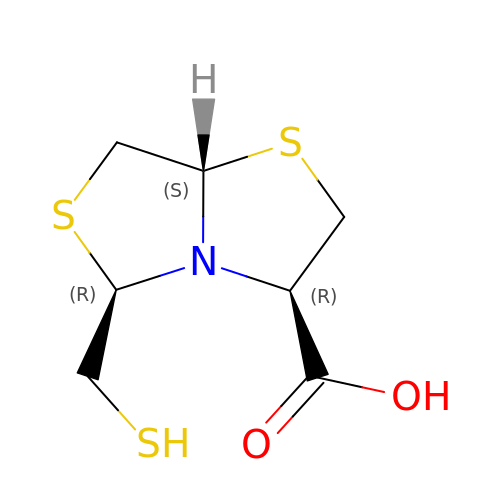(3R,5R,7aS)-5-(sulfanylmethyl)tetrahydro[1,3]thiazolo[4,3-b][1,3]thiazole-3-carboxylic acid | C7 H11 N O2 S3 | ZTWVMVSSSBGFHH-JKUQZMGJSA-N> GSMAHSDGIFKKEQAMCLEKIQRANELMGFNDSSPGCPGMWDNITCWKPAHVGEMVLVSCPELFRI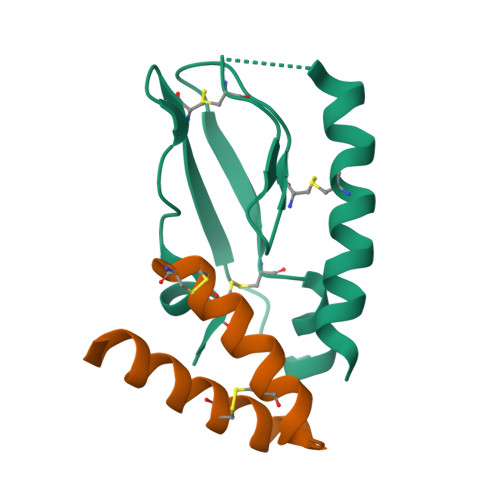FNPDQDMGVVSRNCTEDGWSEPFPHYFDACGFDEYESET;> CDATCQFRKAIDDCARQAYHSSVFKACMKQKKKEWKAGX> MYYESLTKQYPVSKTIRNELIPIGKTLDNIRQNNILESDVKRKQNYEHVKGILDEYHKQLINEALDNCTLPSLKIAAEIYLKNQKEVSDREDFNKTQDLLRKEVVEKLKAHENFTKIGKKDILDLLEKLPSISEDDYNALESFRNFYTYFTSYNKVRENLYSDKEKSSTVAYRLINENFPKFLDNVKSYRFVKTAGILADGLGEEEQDSLFIVETFNKTLTQDGIDTYNSQVGKINSSINLYNQKNQKANGFRKIPKMKMLYKQILSDREESFIDEFQSDEVLIDNVESYGSVLIESLKSSKVSAFFDALRESKGKNVYVKNDLAKTAMSNIVFENWRTFDDLLNQEYDLANENKKKDDKYFEKRQKELKKNKSYSLEHLCNLSEDSCNLIENYIHQISDDIENIIINNETFLRIVINEHDRSRKLAKNRKAVKAIKDFLDSIKVLERELKLINSSGQELEKDLIVYSAHEELLVELKQVDSLYNMTRNYLTKKPFSTEKVKLNFNRSTLLNGWDRNKETDNLGVLLLKDGKYYLGIMNTSANKAFVNPPVAKTEKVFKKVDYKLLPVPNQMLPKVFFAKSNIDFYNPSSEIYSNYKKGTHKKGNMFSLEDCHNLIDFFKESISKHEDWSKFGFKFSDTASYNDISEFYREVEKQGYKLTYTDIDETYINDLIERNELYLFQIYNKDFSMYSKGKLNLHTLYFMMLFDQRNIDDVVYKLNGEAEVFYRPASISEDELIIHKAGEEIKNKNPNRARTKETSTFSYDIVKDKRYSKDKFTLHIPITMNFGVDEVKRFNDAVNSAIRIDENVNVIGIDRGERNLLYVVVIDSKGNILEQISLNSIINKEYDIETDYHALLDEREGGRDKARKDWNTVENIRDLKAGYLSQVVNVVAKLVLKYNAIICLEDLNFGFKRGRQKVEKQVYQKFEKMLIDKLNYLVIDKSREQTSPKELGGALNALQLTSKFKSFKELGKQSGVIYYVPAYLTSKIDPTTGFANLFYMKCENVEKSKRFFDGFDFIRFNALENVFEFGFDYRSFTQRACGINSKWTVCTNGERIIKYRNPDKNNMFDEKVVVVTDEMKNLFEQYKIPYEDGRNVKDMIISNEEAEFYRRLYRLLQQTLQMRNSTSDGTRDYIISPVKNKREAYFNSELSDGSVPKDADANGAYNIARKGLWVLEQIRQKSEGEKINLAMTNAEWLEYAQTHLL

Cas12a is a programmable nuclease for adaptive immunity against invading nucleic acids in CRISPR–Cas systems. Among the Cas12a orthologs, Lachnospiraceae bacterium MA2020 (Lb2) Cas12a is the smallest in molecular weight and recognizes a short spacer (14 nt) for cleavage and the creation of indels with high fidelity. Typically, Cas12a exhibits a bilobed architecture: a recognition lobe (the REC1 and REC2 domains), and a nuclease (NUC) lobe (the WED, PI, RuvC, BH, and Nuc domains) for cleaving nucleic acids. We demonstrate that apo Lb2Cas12a assumes a unique, elongated conformation, whereas the Lb2Cas12a+crRNA binary complex exhibits a compact conformation that subsequently rearranges to a semi-open conformation in the Lb2Cas12a+crRNA+DNA ternary complex.

Of note, the ternary complex contains an RNA–DNA heteroduplex of only 14 bp that mimics the cleaved heteroduplex that would exist in situ; this 14-bp heteroduplex is shorter than the 20-bp heteroduplex used previously to study Cas12a orthologs in target cleavage conformation assays. In our Cas12a+crRNA+DNA ternary complex structure, the REC domain is rotated compared with the binary complex, forcing the REC linker (261Leu–273Ser) toward the 14-bp heteroduplex. The RNA–DNA duplex passes through a central channel formed by the REC and NUC lobes, which results in the expansion of the central channel. Unlike FnCas12a, the REC and NUC lobes in Lb2Cas12a are not connected through a Nuc domain stem (Arg1056–Asn1066), which permits flexibility between these lobes in Lb2Cas12a. The 14-bp heteroduplex is not sufficiently long to stabilize the DNA-REC2 contact through the finger helix (234Lys~244Gln). Consistently, the 14-nt guide strand of crRNA is the minimum length for efficient cleavage of target dsDNA by Lb2Cas12a. Finally, in the ternary complex, the PI domain is rotated by 38° and lies closer to the PAM nucleotides of the dsDNA. PAM is recognized by the conserved PI domain through Lys575 and Lys518. Rearrangement of the hinge region is also observed in the transition from the binary to the ternary complex. Thus, our comparison of the pre-cleavage binary complex with the post-cleavage ternary complex reveals that bilobed movement drives the structural rearrangement of the ternary complex.> MEKDT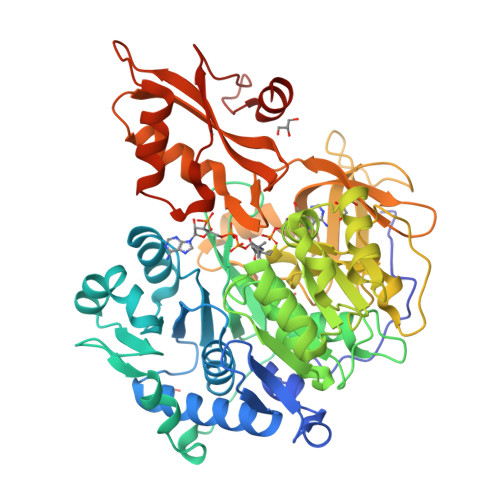KQVDIIFRSKLPDIYIPNHLPLHSYCFENISEFSSRPCLINGANKQIYTYADVELNSRKVAAGLHKQGIQPKDTIMILLPNSPEFVFAFIGASYLGAISTMANPLFTPAEVVKQAKASSAKIIVTQACHVNKVKDYAFENDVKIICIDSAPEGCLHFSVLTQANEHDIPEVEIQPDDVVALPYSSGTTGLPKGVMLTHKGLVTSVAQQVDGENPNLYIHSEDVMLCVLPLFHIYSLNSVLLCGLRVGAAILIMQKFDIVSFLELIQRYKVTIGPFVPPIVLAIAKSPMVDDYDLSSVRTVMSGAAPLGKELEDTVRAKFPNAKLGQGYGMTEAGPVLAMCLAFAKEPFEIKSGACGTVVRNAEMKIVDPKTGNSLPRNQSGEICIRGDQIMKGYLNDPEATARTIDKEGWLYTGDIGYIDDDDELFIVDRLKELIKYKGFQVAPAELEALLLNHPNISDAAVVPMKDEQAGEVPVAFVVRSNGSTITEDEVKDFISKQVIFYKRIKRVFFVDAIPKSPSGKILRKDLRAKLAAGLPN>MDKGSSGKRVIHIGLPELSEEQLIEIGELAQETIIDYVFDHLTRSEVKDIEVTMRINREETLDLEIEVYLEVPIFVKVDVDKLIDEAV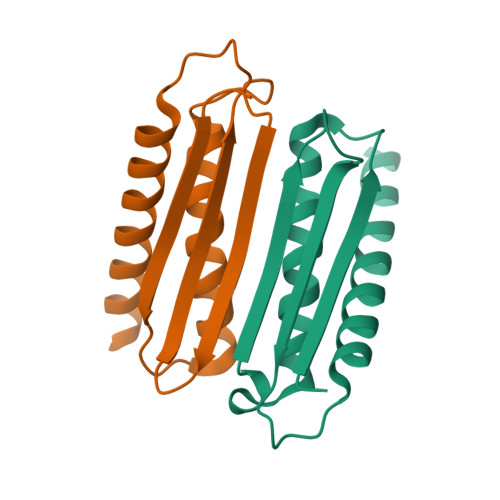ERAYEIVERKLREIANERENQA[6x]>[2x]XA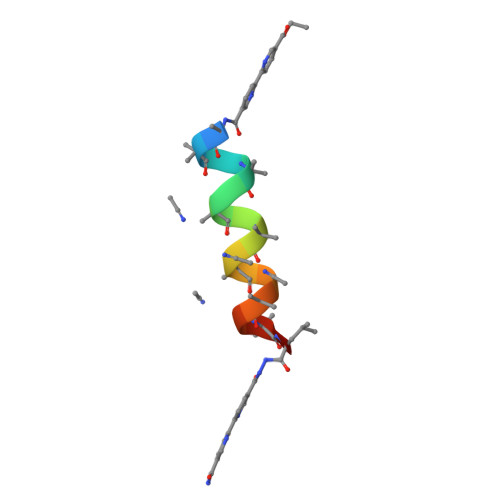AAAAALAAALAQALX> DTETVGGMTLDLPENPPPIPATSTAPSSDSGEVVTATAAQIKELTNYAGVAATAYCRSVVPGTKWDCKQCLKYVPDGKLIKTFTSLLTDTNGFILRSDAQKTIYVTFRGTNSFRSAITDMVFTFTDYSPVKGAKVHAGFLSSYNQVVKDYFPVVQDQLTAYPDYKVIVTGHSLGGAQALLAGMDLYQREKRLSPKNLSIYTVGCPRVGNNAFA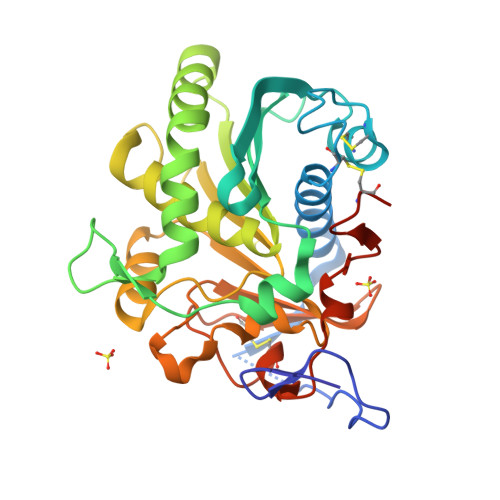YYVDSTGIPFHRTVHKRDIVPHVPPQAFGYLHPGVESWIKEDPADVQICTSNIETKQCSNSIVPFTSIADHLTYFGINEGSCLGSSHHHHHH>[2x]MQLLTNHLGYERLGAKQAILQAQPTLALHHADIICCQSGQSIMQLPLQACGPVAQWHIGDTYSIDFTALNICGDYRIRVGDTESASFCVAEGLLMQNTFSDVLHYFKSQRCSGIYECADKKVPLFGTNETVDVHGGWYDASGDVSKYFSHLSYGNYLNPQQTPMVVWNMLTAYEVLEDEESIADFTRVRLVEEALYGADFLLRMQHPQGYFYMTVFDKWSKSTEQREVCAFSTQDGHKSADYQAGFRQGAGVAIAALAAASRLSNLASTSR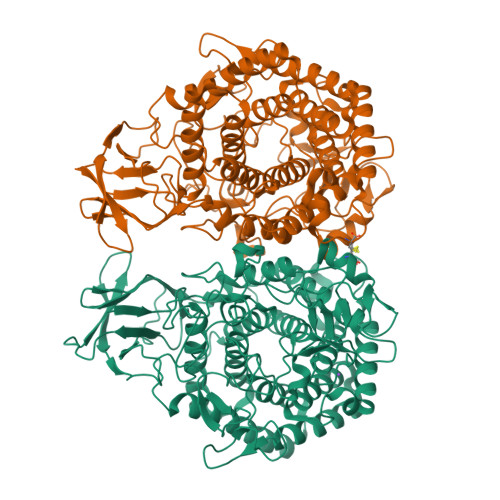IPQCGDIKADTYLEAAKKGYWHLKEMNHQYLDNGKENIIDEYCALLASVELYRSTQENNFLAEARMWADKLMARQMSDHNFAHYWAANDDGSRPYFHAAEAGLPAIALMQYLQIETHAQRAEQCQSVLLNALNFELSITHEVNNPFGYPRQYTKAVNGDKQSAFFMPHDNETGYWWQGENARIASLITMAYMAQNTINDNEIKSQLMIYAHRLTDWILGLNPFDMCMLDGHGRNNPDYLPELGFSNAKGGVCNGITSGFENEQGIAFKPEKQKDDMLQNWRWGEQWIPHGAWYLLAITMQFKERNHVLEHHHHHH> QWNSRYSYNQLKNKDSLIMFLVEIFRSLFVSNCIDKNIDNVLLSIEEMFIDHYYNPQHSRLKYLIDDVGIFFTKLPITKAFHTYNKKYRITKRLYAPPTFNEVRHILNLAQILSLEEGLDLLTFDANETLYPDGHDFNDEVLASYISCLLKKMNIAIVTAASYNNDAEKYQKRLENLLKYFSKHNIKDGSYKNFYVMGGESNYLFKCNEEAT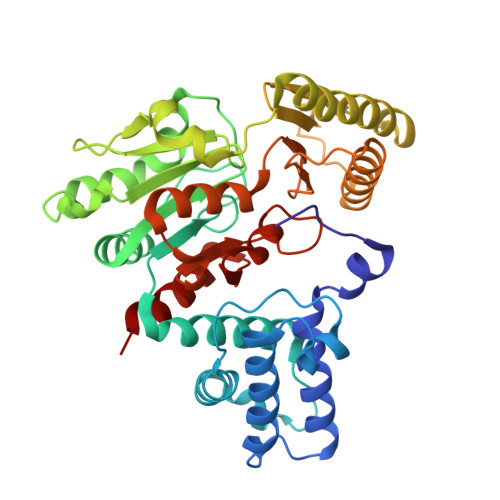LYSVPENEWRHYKKFVDYDTVQEILNISEKCLEKVIKDFGLCAQIQRKEKSIGLVPNKIPSLNIKNEQKNYMIKYEVLEEAVIRIKKEIIKNKITAPYCAFNGGQDLWVDVGNKAEGLLILQKLLKIQKKKCCHIGDQFLHSGNDFPTRFCSLTLWVSNPQETKACLKSIMHLN> QQWFCNSSDAIISYSYCDHLKFPISISSEPCIRLRGTNGFVHVEFIP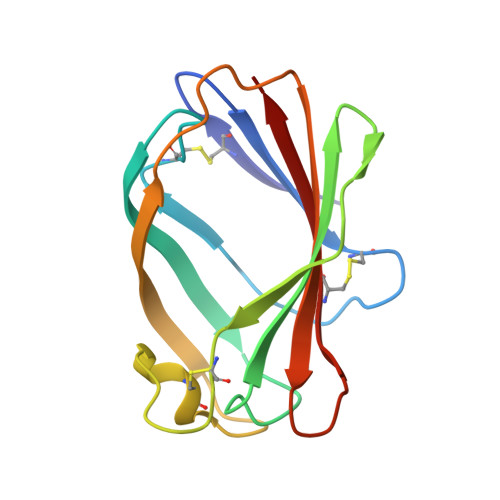RGNLKYLYFNLFISVNSIELPKRKEVLCHGHDDDYSFCRALKGETVNTSIPFSFEGILFPKGHYRCVAEAIAGDTEEKLFCLNFTIIH N-(2-cyano-3-methyl-1H-indol-5-yl)pentane-1-sulfonamide | C15 H19 N3 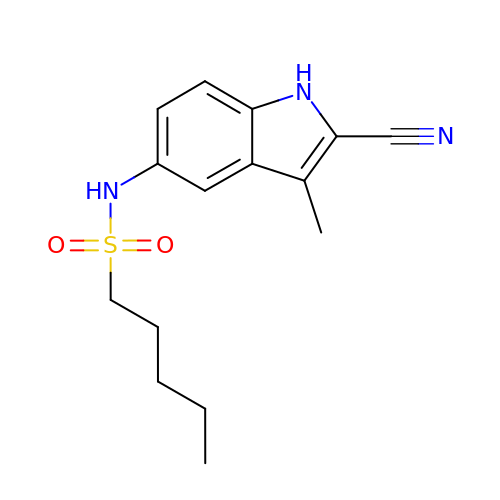O2 S | YSEFPNYCRCSWGW-UHFFFAOYSA-N> MEEHTEAGSAPEMGAQKALIDNPADILVIAAYFLLVIGVGLWSMCRTNRGTVGGYFLAGRSMVWWPVGASLFASNIGSGHFVGLAGTGAASGLAVAGFEWNALFVVLLLGWLFAPVYLTAGVITMPQYLRKRFGGRRIRLYLSVLSLFLYIFTKISVDMFSGAVFIQQALGWNIYASVIALLGITMIYTVTGGLAALMYTDTVQTFVILGGACILMGYAFHEVGGYSGLFDKYLGAATSLTVSEDPAVGNISSFCYRPRPDSYHLLRHPVTGDLPWPALLLGLTIVSGWYWCSDQ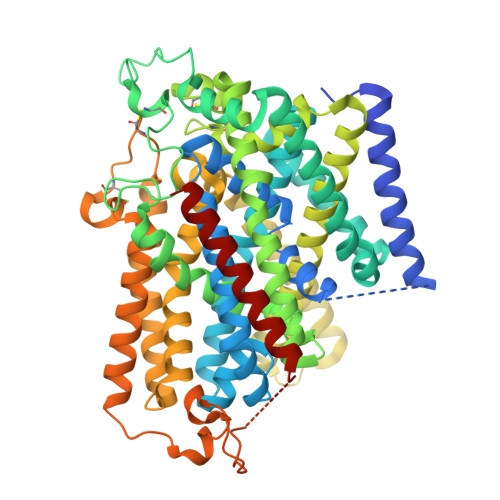VIVQRCLAGKSLTHIKAGCILCGYLKLTPMFLMVMPGMISRILYPDEVACVVPEVCRRVCGTEVGCSNIAYPRLVVKLMPNGLRGLMLAVMLAALMSSLASIFNSSSTLFTMDIYTRLRPRAGDRELLLVGRLWVVFIVVVSVAWLPVVQAAQGGQLFDYIQAVSSYLAPPVSAVFVLALFVPRVNEQGAFWGLIGGLLMGLARLIPEFSFGSGSCVQPSACPAFLCGVHYLYFAIVLFFCSGLLTLTVSLCTAPIPRKHLHRLVFSLRHSKEEREDLDADEQQGSSLPVQNGCPESAMEMNEPQAPAPSLFRQCLLWFCGMSRGGVGSPPPLTQEEAAAAARRLEDISEDPSWARVVNLNALLMMAVAVFLWGFYA>MFEARLVQGSILKKVLEALKDLINEACWDISSSGVNLQSMDSSHVSLVQLTLRSEGFDTYRCDRN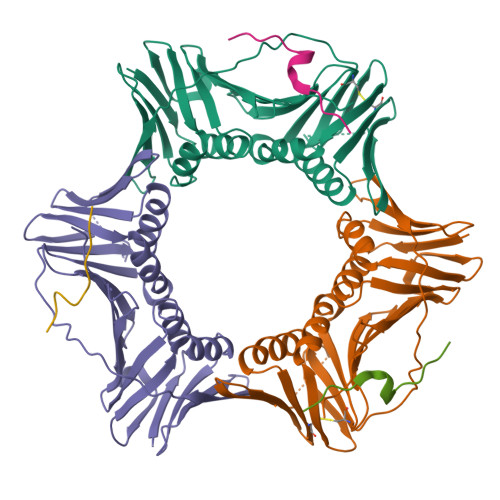LAMGVNLTSMSKILKCAGNEDIITLRAEDNADTLALVFEAPNQEKVSDYEMKLMDLDVEQLGIPEQEYSCVVKMPSGEFARICRDLSHIGDAVVISCAKDGVKFSASGELGNGNIKLSQTSNVDKEEEAVTIEMNEPVQLTFALRYLNFFTKATPLSSTVTLSMSADVPLVVEYKIADMGHLKYYLAPKIEDEEGSLEHHHHHHH[3x];>[3x]SNSHQNVLSNYFPRVS>GAMVPG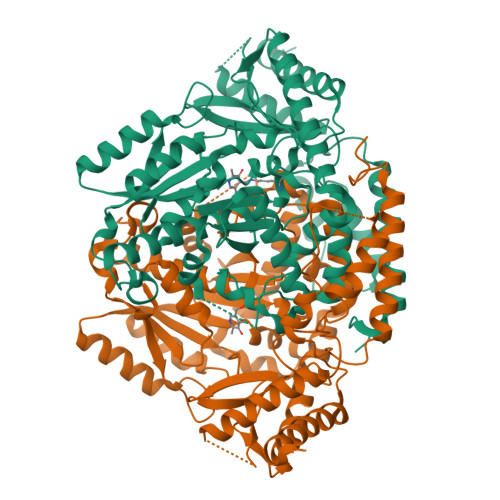SQTSPVSALPPDCGTGNPHDFIFNDHQLSAWARQTEQVLALMTETVKGVEKPFSGILPHELAREFSGVDLDQSLGSNEAALEELKKLYLRDAVWFHHPKYVAHLNCPVVLPSLLAEQIMAAVNSSVDTWDQSAGGTLIEQKVIDWTLSRIGLPAGADGIFTSGGTQSNLMAMLLARDSWCAAHHPGHLIKHRGLPHDAAKWRVFTSKLSHFSIQKSMAILGLGYDAVIPVDYDERYRMDVDCLKQEVQRCLQQGLIPVAVVATSGTTDFGSIDPLGAISELCKHHGMWMHVDAAYGCGLLVSESHRPRLAGIEKADSVTVDYHKSFFQTVSCGAFFVRDKHHLSHVTHHADYLNPLSAQQEGTPNLVNKSIQTTRRFDALKMWLTLRVSGPMALGNAFDDILALTQIAHQLLNAHPAIEVLHVPELTTQIFRYVPRPGMNDALTDEINTNIRKAVFRSGNAVIAGTKVNGRQYLKFTLLNPNTTAADIEDVIALIVHYGREQVRGPAVTTAPL[6x]> MKEEKRSSTGFLVKQRAFLKLYMITMTEQERLYGLKLLEVLRSEFKEIGFKPNHTEVYRSLHELLDDGILKQIKVKKEGAKLQEVVL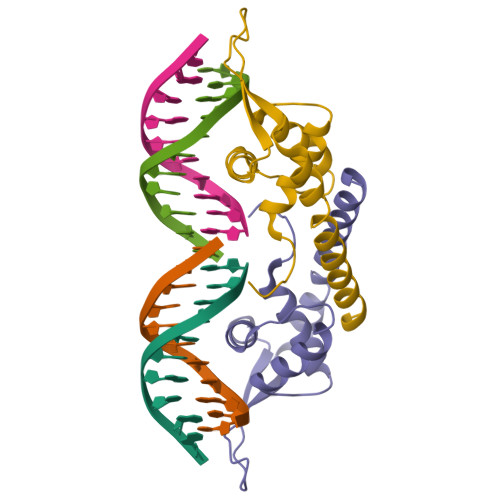YQFKDYEAAKLYKKQLKVELDRSKKLIEKALSDNF>[4x]HPETLVKVKDAEDQLGARVGYIELDLNSGKILESFRPEERFPMMSTFKV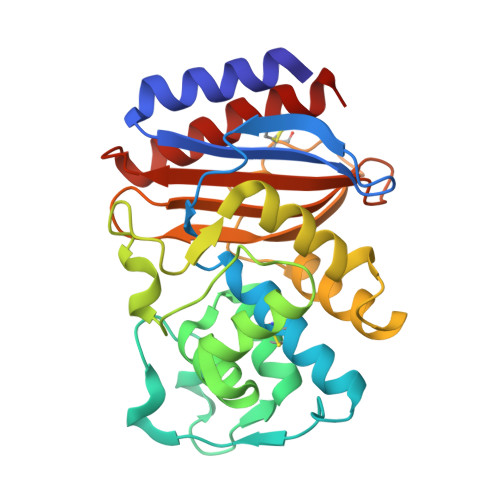LLCGAVLSRVDAGQEQLGRRIHYSQNDLVEYSPVTEKHLTDGMTVRELCSAAITMSDNTAANLLLTTIGGPKELTAFLHNMGDHVTRLDRWEPELNEAIPNDERDTTTPAAMATTLRKLLTGELLTLASRQQLIDWMEADKVAGPLLRSCLPAGWFIADKSGAGERGSRGIIAALGPDGKPSRIVVIYTTGSQATMDERNRQIAEICASLIKHW Here, we characterize the O-methyltransferases BelI and CysG, which catalyze the initial step of β-lactone formation. Employing techniques such as crystallography, computational analysis, mutagenesis, and activity assays, we identified a His-His-Asp (HHD) motif in the active sites of the two enzymes, which is crucial for binding a catalytically active calcium ion. As expected, BelI as well as CysGΔN16 adopt the class I methyltransferase Rossmann fold, characterized by a core domain of a seven-stranded β-sheet flanked by α-helices. The HHD-motif enables regiospecific C1-carboxy group methylation of their respective malic substrates.

Notably, the N-terminally truncated CysGΔN16 variant was active with metal ions available but inactive in the presence of EDTA. Indeed, the 2Fo-Fc electron density map displayed the structural integrity of the enzyme in a metal-free state. Thus, we conclude that the divalent metal ion is crucial for the catalytic function of CysG rather than for structural stability.

>[2x]GSTYDALRRQLIPSFDLLYGSAVSVVAMSVPATARILDLGAGTGLLGAALRERLPDAELLLQDRSQAMLEQARQRFADDDQVAIRVADHLDELPAGPFDAVVSALSIHHLEHQDKQDLFTRIRKILRPGGIFVNVEQVLAPTSELEKMYDRQHEAHVLASDTPAEEWAAGRERMKHDIPIDVETQIQWLRDAGFTTADCLAKDWRFATYAGWNGS> SLQFLL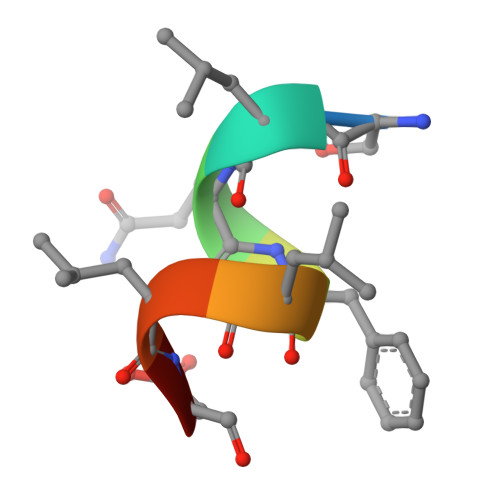DT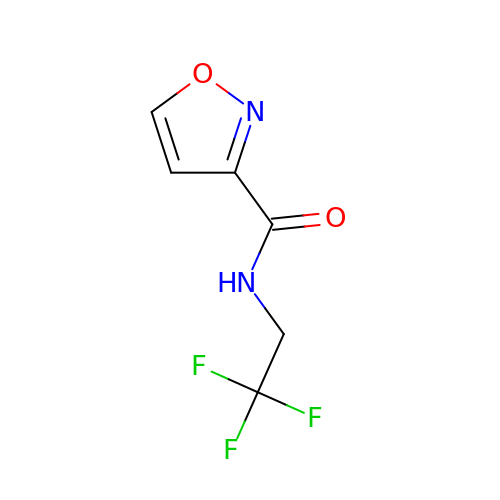N-(2,2,2-trifluoroethyl)-1,2-oxazole-3-carboxamide | C6 H5 F3 N2 O2 | OOPKAKDUIYDDGZ-UHFFFAOYSA-N>[2x]QTQVLFEHPLNEKMRTWLRIEFLIQQLTVNLPIVDHAGALHFFRNVSELLDVFERGEVRTELLKELDRQQRKLQTWIGVPGVDQSRIEALIQQLKAAGSVLISAPRIGQFLREDRLIALVRQRLSIPGGCCSF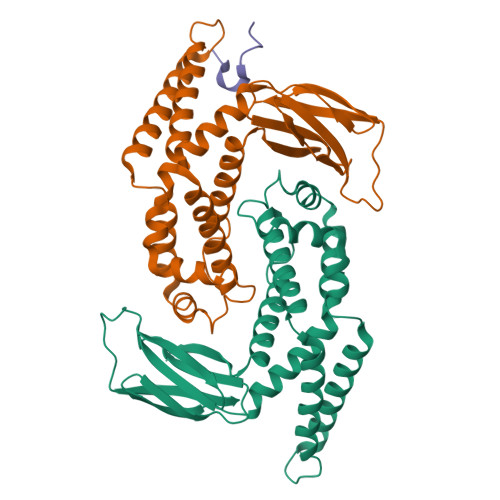DLPTLHIWLHLPQAQRDSQVETWIASLNPLTQALTMVLDLIRQSAPFRKQTSLNGFYQDNGGDADLLRLNLSLDSQLYPQISGHKSRFAIRFMPLDSENGQVPERLDFELACC;> DYLDIPAFLRKQ>[2x]KQGPTSVAYVEVNNNSMLNVGKYTLADGGGNAFDVAVIFAANINYDTGTKTAYLHFNENVQRVLDNAVTQIRPLQQQGIKVLLSVLGNHQGAGFANFPSQQ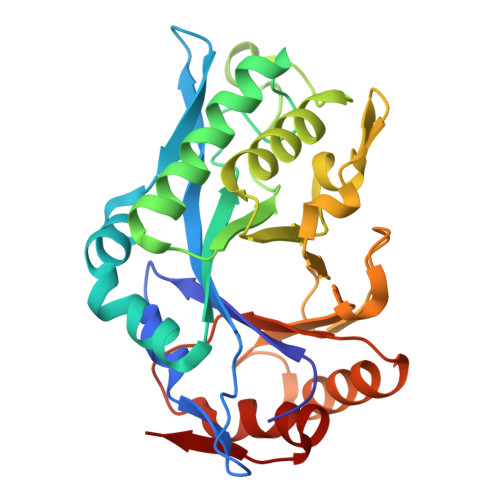AASAFAKQLSDAVAKYGLDGVDFDDQYAEYGNNGTAQPNDSSFVHLVTALRANMPDKIISLYNIGPAASRLSYGGVDVSDKFDYAWNPYYGTWQVPGIALPKAQLSPAAVEIGRTSRSTVADLARRTVDEGYGVYLTYNLDGGDRTADVSAFTRELYGSEAVRT> MGSYLHEPPGDEPSMRIEQPKTADRAPEQVAIHICEPSKVVTESFPFSETAEPEAKSKNCPCPEIARIGPCPNKPPKIPINRGLSRISTNKSRPKSRFGEPSWPVESSLDLTSQSPVSPYREEAFSVENCGTAGSRRGSFARGTTSRAASSSRKDETKEGPDEKEVYQRVTAQLSARNQKRMTVKLMIELSVFLCLLGCLVCSLTVDGFKRYTVIGLDIWKWFLLLLVIFSGMLITHWIVHVAVFFVEWKFLMRKNVLYFTHGLKTSVEVFIWITVVLATWVMLIKPDVNQPHQTRKILEFVTWTIVTVLIGAFLWLVKTTLLKILASSFHLNRFFDRIQESVFHHSVLQTLAGRPVVELAQGISRTESQDGAGQVSFMEHTKTQNKKVVDVGKLHQMKQEKVPAWTMQLLVDVVSNSGLSTMSGMLDEDMVEGGVELDDDEITNEEQAIATAVRIFDNIVQDKVDQSYIDRVDLHRFLIWEEVDHLFPLFEVNEKGQISLKAFAKWVVKVYNDQAALKHALNDNKTAVKQLNKLVTAILIVMMIVIWLIVTGIATTKLIVLLSSQLVVAAFIFGNTCKTIFEAIIFVFVMHPFDVGDRCVIDGNKMLVEEMNILTTVFLKWDKEKVYYPNSILCTKAIGNFFRSPDQGDVLEFSVDFTTPVLKIGDLKDRIKMYLEQNLNFWHPQHNMVVKEIENVNKIKMALFVNHTINFQDFAEKNRRRSELVLELKKIFEELDIKYNLLPQEISIRNMGSGSLEVLFQ

Flycatcher1 (FLYC1), a MscS homolog, has recently been identified as a candidate mechanosensitive (MS) ion channel involved in Venus flytrap prey recognition. FLYC1 is an ortholog of prokaryotic MS ion channel MscS (mechanosensitive ion channel of small conductance), which functions as an osmotic release valve, and is perhaps the most extensively studied MS channel. FLYC1 comprises a homoheptamer with six TMs (TM1–TM6) per protomer and intracellular N and C termini. A glycine-containing hinge (G575) splits TM6 into two halves (TM6a and TM6b), and the β-rich C-termini of the FLYC1 protomers come together to form a hollow cytoplasmic cage.

A striking difference between the classes is the conformation of the cytosolic TM4-TM5 linker, which can be in an up or down conformation. In the up conformation, the TM4-TM5 linker is parallel to the membrane plane, while in the down conformation, the linker swivels towards the cytosol. TM1-TM5 are displaced in a clockwise manner in the down state compared to the up state when viewed from the extracellular side. In the down state, a short six-residue coil (P96-S101) from the N-terminus interacts near the side portals of the cytoplasmic vestibule. Symmetry expansion followed by variability analysis in cryoSPARC40 confirmed the presence of density for this short peptide only in the down conformation. In the down state, R334 shifts upward and does not contact D598. TM6a hinges away from the pore center in the down state, which displaces F572 outward. Therefore, the distinct TM6 conformations in up and down states could represent different functional states. 3D EM variability analysis displayed a lipid-like density at the top of the pore, which differs from the ‘hook’ and pore lipids of EcMscS, as it is not on the outer side of TM6a or in the middle of the pore, respectively, but rather it intercalates in-between adjacent TM6a helices. This density is associated with the down class, but it only appears when the adjacent subunit (clockwise when viewed from extracellular side) is positioned far enough to create a side opening to the membrane.>[2x]PVNPCCYYPCQHQGICVRFGLDRYQCDCTRTGYSGPNCTIPEIWTWLRTTLRPSPSFIHFLLTHGRWLWDFVNATFIRDTLMRLVLTVRSNLIPSPPTYNIAHDYISWESFSNVSYYTRILPSVPRDCPTPMGTKGKKQLPDAEFLSRRFLLRRKFIPDPQGTNLMFAFFAQHFTHQFFKTSGKMGPGFTKALGHGVDLGHIYGDNLERQYQLRLFKDGKLKYQMLNGEVYPPSVEEAPVLMHYPRGIPPQSQMAVGQEVFGLLPGLMLYATIWLREHNRVCDLLKAEHPTWG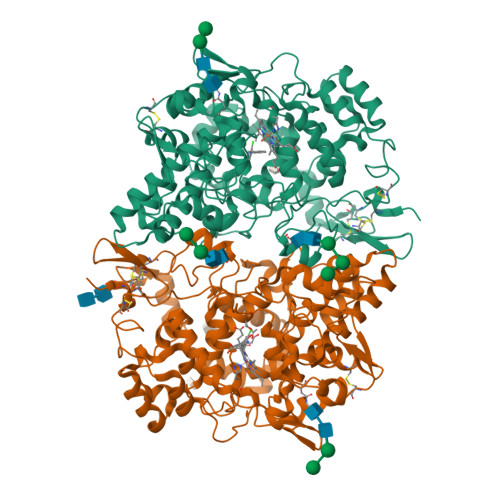DEQLFQTARLILIGETIKIVIEEYVQQLSGYFLQLKFDPELLFGAQFQYRNRIAMEFNQLYHWHPLMPDSFRVGPQDYSYEQFLFNTSMLVDYGVEALVDAFSRQPAGRIGGGRNIDHHILHVAVDVIKESRVLRLQPFNEYRKRFGMKPYTSFQELTGEKEMAAELEELYGDIDALEFYPGLLLEKCHPNSIFGESMIEMGAPFSLKGLLGNPICSPEYWKASTFGGEVGFNLVKTATLKKLVCLNTKTCPYVSFHVPD> AMMNAFKEITTMADRINLPR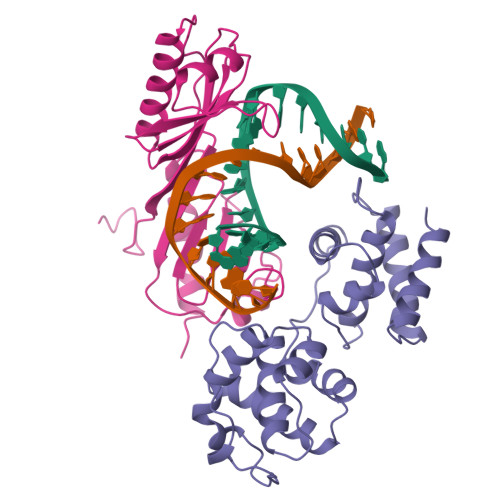NKVDRTNNLFRQAYEQKSLKGRANDAIASACLYIACRQEGVPRTFKEICAVSRISKKEIGRCFKLILKALETSVDLITTGDFMSRFCSNLCLPKQVQMAATHIARKAVELDLVPGRSPISVAAAAIYMASQASAEKRTQKEIGDIAGVADVTIRQSYRLIYPRAPDLFPTDFKFDTPVDKLPQL;> MTDQGLEGSNPVDLSKHPSGIVPTLQNIVSTVNLDCKLDLKAIALQARNAEYNPKRFAAVIMRIREPKTTALIFASGKMVCTGAKSEDFSKMAARKYARIVQKLGFPAKFKDFKIQNIVGSCDVKFPIRLEGLAYSHAAFSSYEPELFPGLIYRMKVPKIVLLIFVSGKIVITGAKMRDETYKAFENIYPVLSEFRKIQQ Promoter escape requires positive transcription elongation factor b (P-TEFb), a heterodimeric protein kinase composed of CDK9 and cyclin T1 (CycT1) subunits. P-TEFb triggers promoter escape by directly or indirectly stimulating phosphorylation of the RNA polymerase II C-terminal domain and the associated factors, NELF (negative elongation factor) and DSIF (DRB sensitivity inducing factor). Recent studies of gene fusions in myeloid leukemias, as well as complexes recruited to the HIV promoter by the HIV Tat protein, uncovered a family of Super Elongation Complexes (SECs) that bring together active P-TEFb and other transcription elongation factors. AFF4 is an intrinsically disordered scaffold that binds partners via 20–50 residue segments.

Here, we report the structural and functional analysis of P-TEFb in complex with the cognate binding site on the SEC scaffold protein, AFF4. In all three independent copies of the complex in the crystals, AFF4 residues Leu34-Ile66 are ordered, binding to the second cyclin domain of CycT1 opposite CDK9. In one complex, an isolated helix containing AFF4 residues 3–21 bridges symmetry-related CDK9 molecules in the crystals. Consistent with the coupling of folding to binding, AFF4 lacks intramolecular tertiary contacts as it snakes across the CycT1 surface. An extended segment in AFF4 tracks antiparallel to the H3′-H4′ loop in CycT1, and two short AFF4 helices fit into shallow grooves in CycT1 between H3′ and H5′ and the surface formed by H2′ and H3′. Compared to the separated models, 1457 Å2 of AFF4 and 1251 Å2 of CycT1 accessible surface are buried in the complex. A pocket between CycT1 Leu163-Val164-Arg165, Trp221, and Tyr224, for example, anchors AFF4 Phe35, which forms a classic edge-to-face interaction with the Tyr. CycT1 Trp210 adjusts to create a site that buries AFF4 Pro38 and allows a short antiparallel β-sheet to form between AFF4 Tyr39-Val41 and CycT1 Asn 209-Glu211. To accommodate AFF4, helix H5′ straightens and residues 251–256 form a helical segment that packs against CycT1 helices H1 and H2' and forms part of the AFF4 binding surface. Superposition of the CycT1 subunits of the structures of Tat-P-TEFb and AFF4-P-TEFb shows that Tat is positioned to pack against helix 2 of AFF4.

>GHMAKQYDSVECPFCDEVSKYEKLAKIGQGTFGEVFKARHRKTGQKVALKKVLMENEKEGFPITALREIKILQLLKHENVVNLIEICRTKASPYNRCKGSIYLVFDFCEHDLAGLLSNVLVKFTLSEIKRVMQMLLNGLYYIHRNKILHRDMKAANVLITRDGVLKLADFGLARAFSLAKNSQPNRYTNRVVTLWYRPPELLLGERDYGPPIDLWGAGCIMAEMWTRSPIMQGNTEQHQLALISQLCGSITPEVWPNVDNYELYEKLELVKGQKRKVKDRLKAYVRDPYALDLIDKLLVLDPAQRIDSDDALNHDFFWSDPMPSDLKGMLST[3x];>MEGERKNNNKRWYFTREQLENSPSRRFGVDPDKELSYRQQAANLLQDMGQRLNVSQLTINTAIVYMHRFYMIQSFTQFPGNSVAPAALFLAAKVEEQPKKLEHVIKVAHTCLHPQESLPDTRSEAYLQQVQDLVILESIILQTLGFELTIDHPHTHVVKCTQLVRASKDLAQTSYFMATNSLHLTTFSLQYTPPVVACVCIHLACKWSNWEIPVSTDGKHWWEYVDATVTLELLDELTHEFLQILEKTPNRLKRIWNWRACEAA[3x];>SNANREDRNVLRMKERERRNQEIQQGEDAFPPSSPLFAEPYKVTSKEDKLSSRIQSMLGNYDEMKDFIGDRSIPK[3x]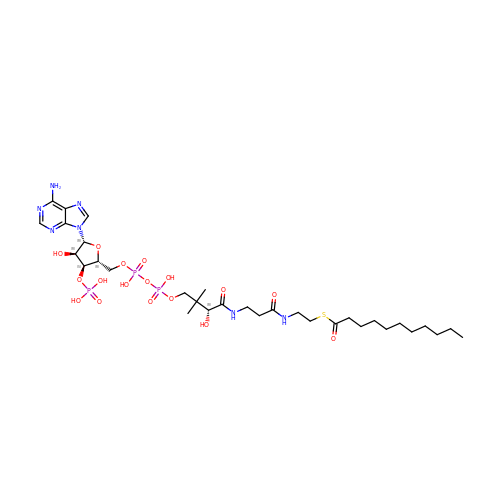S-{(3S,5R,9R)-1-[(2R,3S,4R,5R)-5-(6-amino-9H-purin-9-yl)-4-hydroxy-3-(phosphonooxy)tetrahydrofuran-2-yl]-3,5,9-trihydroxy-8,8-dimethyl-3,5-dioxido-10,14-dioxo-2,4,6-trioxa-11,15-diaza-3lambda~5~,5lambda~5~-diphosphaheptadecan-17-yl} undecanethioate | C32 H56 N7 O17 P3 S | IZWCGXGZGYKDHR-GRBGHKMPSA-N>MGHHHHHHSSPKIEERTYPPQIPAQQELGDFSAYQSVLPEPLRKAEKLLQETGIKESTKTNTLKKLLRFSVEAGGLTEENVVGKLQEILCDMLPSADKWQEPIHSKYIVLFGSTG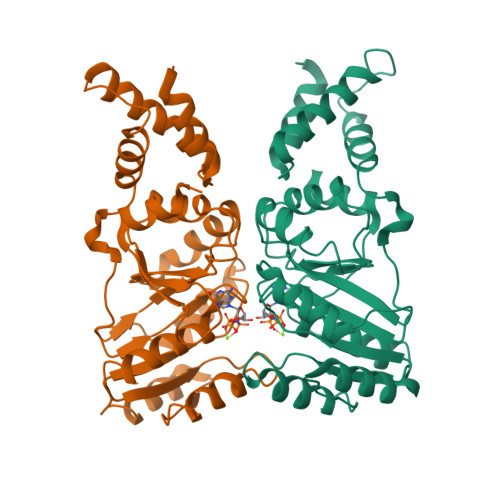AGKTTTLAKLAAISMLEKHKKIAFITTDTYRIAAVEQLKTYAELLQAPLEVCYTKEEFQQAKELFSEYDHVFVDTAGRNFKDPQYIDELKETIPFESSIQSFLVLSATAKYEDMKHIVKRFSSVPVNQYIFTKIDETTSLGSVFNILAESKIGVGFMTNGQNVPEDIQTVSPLGFVRMLCR[8x]>[6x]AMGNKLFNIAQRILDTNSVLLTERGDYIVWINNSWKFNSEEPLITKLILSIRHQLPKEYSSELLCP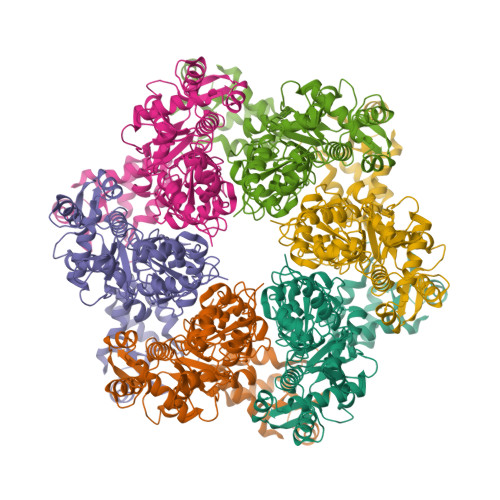RKRKTVEANIRDMLVDSVETDTYPDKLPFKNGVLDLVDGMFYSGDDAKKYTCTVSTGFKFDDTKFVEDSPEMEELMNIINDIQPLTDENKKNRELYEKTLSSCLCGATKGCLTFFFGETATGKSTTKRLLKSAIGDLFVETGQTILTDVLDKGPNPFIANMHLKRSVFCSELPDFACSGSKKIRSDNIKKLTEPCVIGRPCFSNKINNRNHATIIIDTNYKPVFDRIDNALMRRIAVVRFRTHFSQPSGREAAENNDAYDKVKLLDEGLDGKIQNNRYRFAFLYLLVKWYKKYHVPIMKLYPTPEEIPDFAFYLKIGTLLVSSSVKHIPLMTDLSKKGYILYDNVVTLPLTTFQQKISKYFNSRLFGHDIESFINRHKKFANVSDEYLQYIFIEDISSP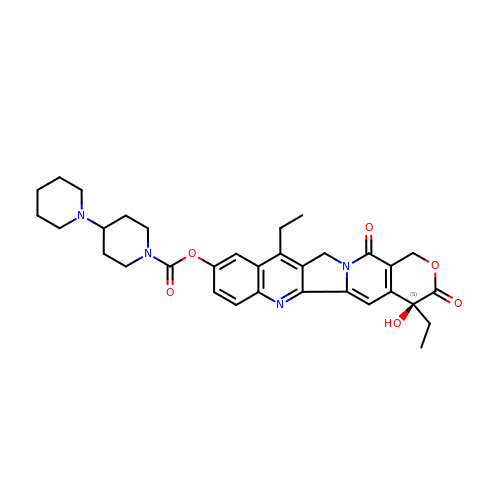(4S)-4,11-DIETHYL-4-HYDROXY-3,14-DIOXO-3,4,12,14-TETRAHYDRO-1H-PYRANO[3',4':6,7]INDOLIZINO[1,2-B]QUINOLIN-9-YL 1,4'-BIPIPERIDINE-1'-CARBOXYLATE | C33 H38 N4 O6 | UWKQSNNFCGGAFS-XIFFEERXSA-N methyl (8R)-8-{[(4P)-6-amino-3H-purin-3-yl]methyl}-4-hydroxy-6-(5,6,7-trimethoxy-1H-indole-2-carbonyl)-3,6,7,8-tetrahydropyrrolo[3,2-e]indole-2-carboxylate | C30 H28 N8 O7 | 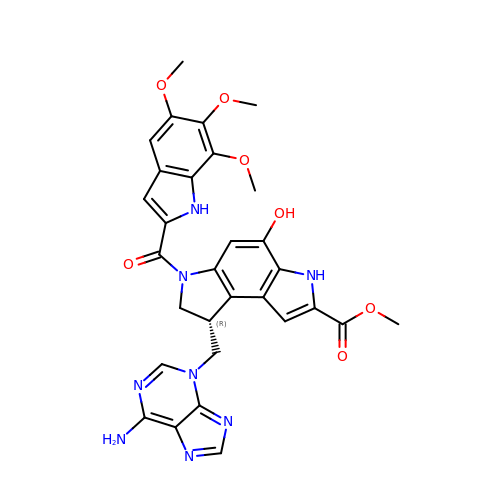AZHBDEJKEVQJNC-CQSZACIVSA-N> AAAAAAAAAAAAAAAAAAAAAAAAAAAA;> GGGUACUC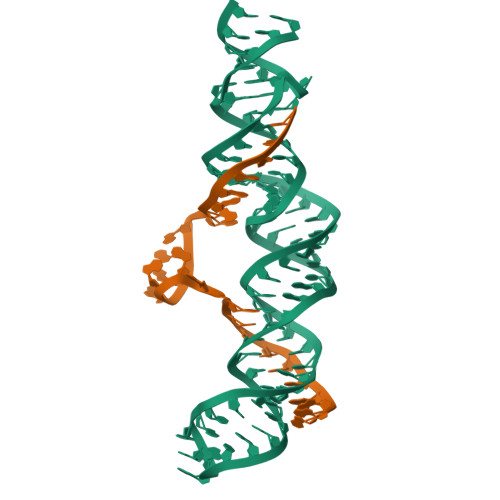UUUUCUUUGUCAUGGUUUUCUCAGGCGAAAGUCUGAGUUUUUACAUGACAAAGUUUUUAACGAGGCCC>[2x]GSYAEGQRKRRNTIHEFKKSAKTTLIKIDPALKIKTKKVNTADQCANRCTRNKGLPFTCKAFVFDKARKQCLWFPFNSMSSGV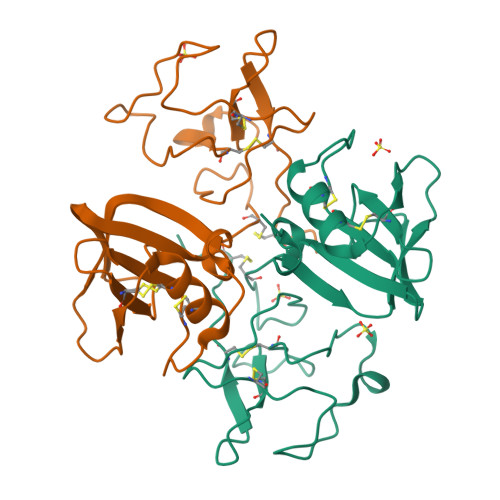KKEFGHEFDLYENKDYIRNCIIGKGRSYKGTVSITKSGIKCQPWSSMIPHEHSFLPSSYRGKDLQENYCRNPRGEEGGPWCFTSNPEVRYEVCDIPQCSEV> ACTKNAIAQTGFNKDKYFNGDVWYVTDYLDLEPDDVPKRYCAALAAGTASGKLKEALYHYDPKTQDTFYDVSELQVESLGKYTANFKKVDKNGNVKVAVTAGNYYTFTVMYADDSSALIHTCLHKGNKAAGDLYAVLNRNKDAAAGDKVKSAVS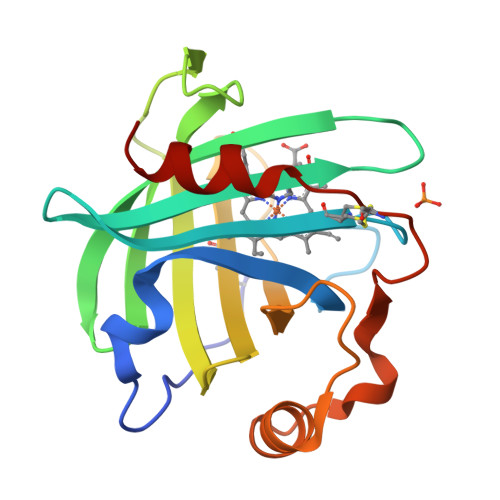AATLEFSKFISTKENNCAYDNDSLKSLLTK>MSIKDSIGLRIKTERECQQMSREVLCLDGAELTVRQLIRIEKGESLPSLDKLSYIAKRLGKSMADLLDHDRIEIPDTYYEMKNRLIKFPTYGDKERVKQKLDLIEDVYNQFFDILPEEELLTLDILENILSFTSWEERPKVEEIYEDLFEQVKRKKKFSTNDLLVIDYYFYHLYGRKQYDKKIFDRIVDRVLKQNIPTDDAYNIALFNDLMAIAGLKISLESFKDFLTVIDKLLAVIEKSQFHSYKPGVYILEAKYELIHNGNKKKATENYDKAIMFASVLEDSV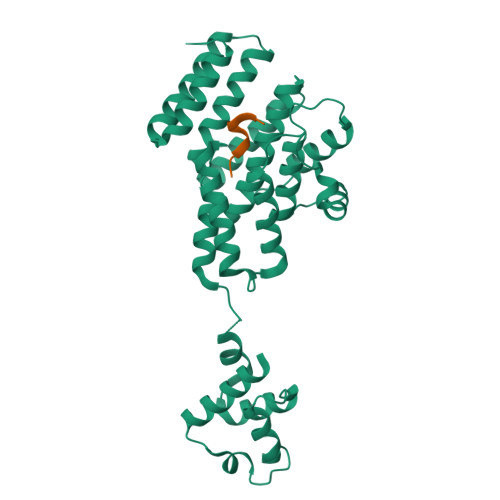LEEKTRAEKAADGLGAGWSHPQFEK[2x];>VPFFMIYY[2x]> MAGDPMGSKNESTASKASGTASEKKKIEYLDKTYEVTVPTDKIAITGSVESMEDAKLLDVHPQGAISFSGKFPDMFKDITDKAEPTGEKMEPNIEKILEMKPDVILASTKFPEKTLQKISTAGTTIPVSHISSNWKENMMLLAQLTGKEKKAKKIIADYEQDLKEIKTKINDKAKDSKAL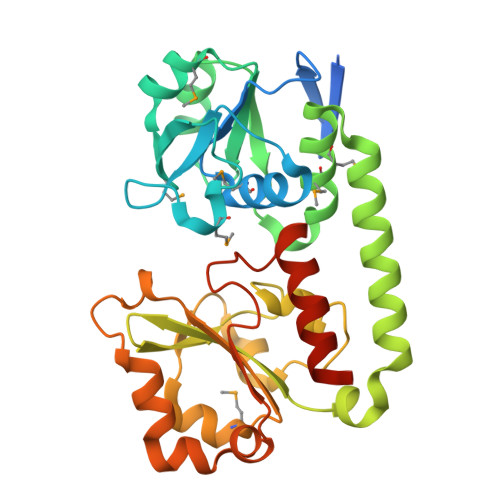VIRIRQGNIYIYPEQVYFNSTLYGDLGLKAPNEVKAAKAQELSSLEKLSEMNPDHIFVQFSDDENADKPDALKDLEKNPIWKSLKAVKEDHVYVNSVDPLAQGGTAWSKVRFLKAAAEKLTQNLEHHHHHH> MSAE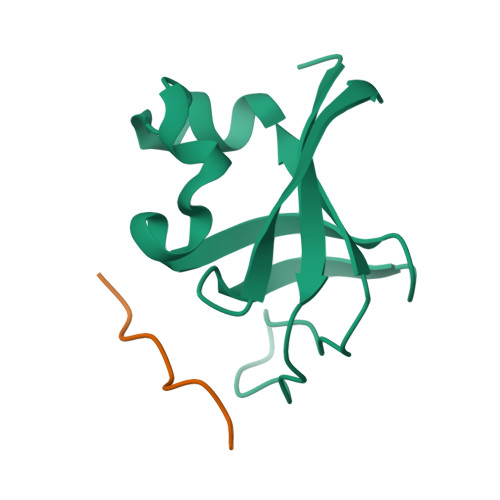GYQYRALYDYKKEREEDIDLHLGDILTVNKGSLVALGFSDGQEARPEEIGWLNGYNETTGERGDFPGTYVEYIGRKKIS;> HSKRPLPPLPSL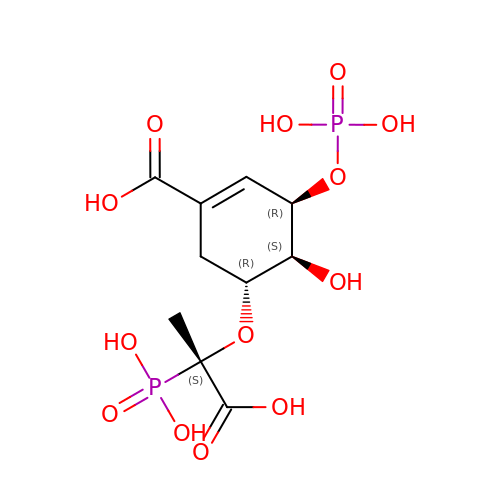[3R-[3A,4A,5B(S*)]]-5-(1-CARBOXY-1-PHOSPHONOETHOXY)-4-HYDROXY-3-(PHOSPHONOOXY)-1-CYCLOHEXENE-1-CARBOXYLIC ACID | C10 H16 O13 P2 | HUOJJMMXOWLGJU-JQCUSGDOSA-N> MSLGAKPFGEKKFIEIKGRRMAYIDEGTGDPILFQHGNPTSSYLWRNIMPHCAGLGRLIACDLIGMGDSDKLDPSGPERYTYAEHRDYLDALWEALDLGDRVVLVVHDWGSVLGFDWARRHRERVQGIAYMEAVTMPLE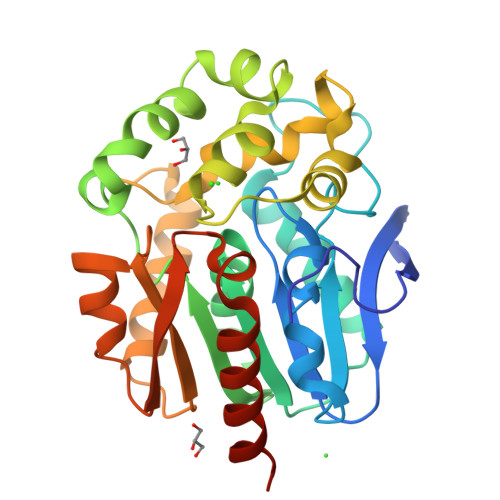WADFPEQDRDLFQAFRSQAGEELVLQDNVFVEQVLPGLILRPLSEAEMAAYREPFLAAGEARRPTLSWPRQIPIAGTPADVVAIARDYAGWLSESPIPKLFINAEPGALTTGRIRDFCRTWPNQTEITVAGAHFIQEDSPDEIGAAIAAFVRRLRPAHHHHHH>STAGKVIKCKAAVLWEEKKPFSIEEVEVAPPKAHEVRIKMVATGICRSDDHVVSGTLVTPLPVIAGHEAAGIVESIGEGVTTVRPGDKVIPLFTPQCGKCRVCKHPEGNFCLKNDLSMPRGTMQDGTSRFTCRGKPIHHFLGTSTFSQYTVVDEISVAKIDAASPLEKVCLIGCGFSTGYGSAVKVAKVTQGSTCAVFGLGGVGLSVIMGCKAAGAARIFGVDINKDKFAKAKEVGATECVNPQDYKKPIQEVLTEMSNGGVDFSFEVIGRLDTMVTALSCCQEAYGVSVIVGVPPDSQNLSMNPMLLLSGRTWKGAIFGGFKSKDSVPKLVADFMAKKFALDPLITHVLPFEKINEGFDLLRSGESIRT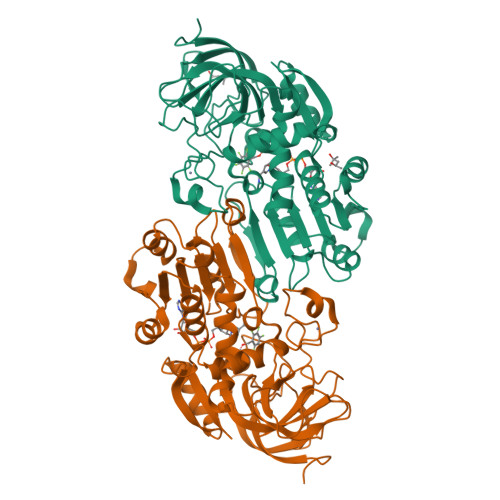ILTF[2x]> MIIWPSYIDKKKSRREGRKVPEELAIEKPSLKDIEKALKKLGLEPKIYRDKRYPRQHWEIAGRVEVDYKGNK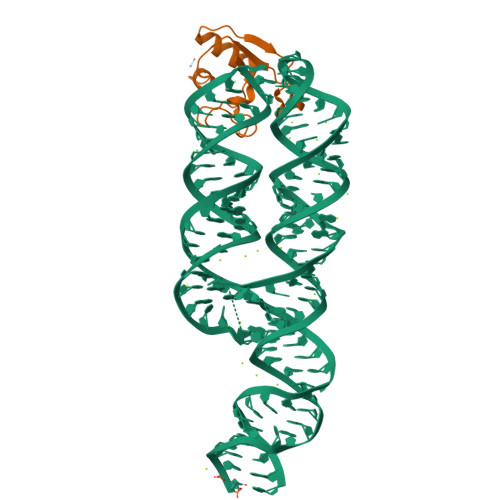LCLLKEIAKIIKGKN> HGSMETPPSRVYGCFLEGPENPKSAACKAAVAAGGTQALYDWNGVNQGNANGNHQAVVPDGQLCGAGKALFKGLNLARSDWPSTAIAPDASGNFQFVYKASAPHATRYFDFYITKDGYNPEKPLAWSDLEPAPFCSITSVKLENGTYRMNCPLPQGKTGKHVIYNVWQRSDSPEAFYACIDVSFSGAVANPWQALGNLRAQQDLPAGATVTLRLFDAQGRDAQRHSLTLAQGANGAKQWPLALAQKVNQDSTLVNIGVLDAYGAVSPVASSQDNQVYVRQAGYRFQVDIELPVEGGGEQPGGDGKVDFDYPQGLQQYDAGTVVRGADGKRYQCKPYPNSGWCKGWDLYYAPGKGMAWQDAWTLLHHHHHHHHHH

Pseudomonas aeruginosa secretes diverse proteins via its type 2 secretion system, including a 39 kDa chitin-binding protein, CbpD. CbpD has recently been shown to be a lytic polysaccharide monooxygenase active on chitin and to contribute substantially to virulence. LPMOs are further characterized by a solvent-exposed Peisach–Blumberg type 2 copper active site in which a mononuclear copper ion is coordinated in a T-shape by a histidine brace comprising the N-terminal amine and two histidines.

Residues 297–374 (the remainder of the linker and the CBM73 domain) were not visible in the electron-density map. All LPMOs have the Glu (sometimes Gln) which is required for enzymatic activity, likely by coordinating H2O2 and reactive oxygen species intermediates. CbpD contains an analogous amino-acid pair Asn46–Glu174, but notably the two amino acids are swapped, a feature that is also present in CjLPMO10A. The maintenance of the polar interaction between the side chains and the proximity of Glu174 to the active site imply that Glu174/Asn46 may also gate the access of cosubstrates or electron donors to the active site when CbpD is bound to crystalline chitin.> MHHHHHHENLYFQSAKLAASNQFGIPNQTDVFAVD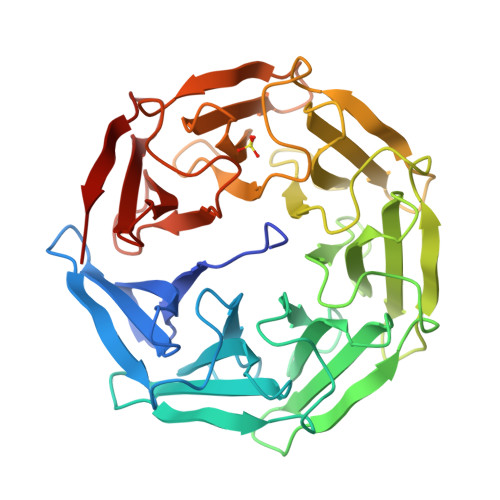GNGSLRVSWVVSAGAWNGPAQIGPAGLFPSRAAVASSNQFGIPNQTDVFAVGRDGALNVAWVVSADRWNGPTPISAAGLFPAGAAIAASNQFGIPNQTDVFAVSDSGALNVAWVVSAERWNGPIPISAAGHFPAGAPLATSNQFGIPNQTDVFVVDNKGALNVAWVVGAGSWNGPIPISPPGLFPPGAAVAASNQFGIPNQTDVFVVDNQGALNVAWVVGADRWNGPVPISPAGLFPPGAAVAASNQFGIPNQTDVFAVGRDGALRVAWVVSAGNWNGPVSISPTNLFPSGAAVAASNQFGIPNQTDVFAADSDGVLHVAWVVSAGNWNGPISIA>[4x]MSESPMFAANGMPKVNQGAEEDVRILGYDPLASPALLQVQIPATPTSLETAKRGRREAIDIITGKDDRVLVIVGPCSIHDLEAAQEYALRLK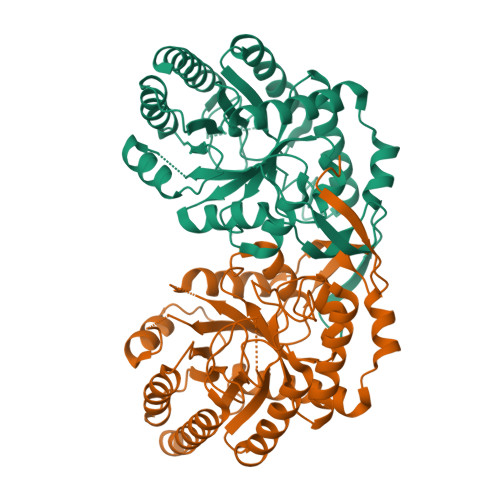KLSDELKGDLSIIMRAYLEKPRTTVGWKGLINDPDVNNTFNINKGLQSARQLFVNLTNIGLPIGSEMLDTISPQYLADLVSFGAIGARTTESQLHRELASGLSFPVGFKNGTDGTLNVAVDACQAAAHSHHFMGVTKHGVAAITTTKGNEHCFVILRGGKKGTNYDAKSVAEAKAQLPAGSNGLMIDYSHGNSNKDFRNQPKVNDVVCEQIANGENAITGVMIESNINEGNQGIPAEGKAGLKYGVSITDACIGWETTEDVLRKLAAAVRQRREVNKK>MRGSHHHHHHGSDQVSLGVVGIGKIARDQHLPAIDAEPGFKLTACASRHAEVTGVRNYRDLRALLAAERELDAV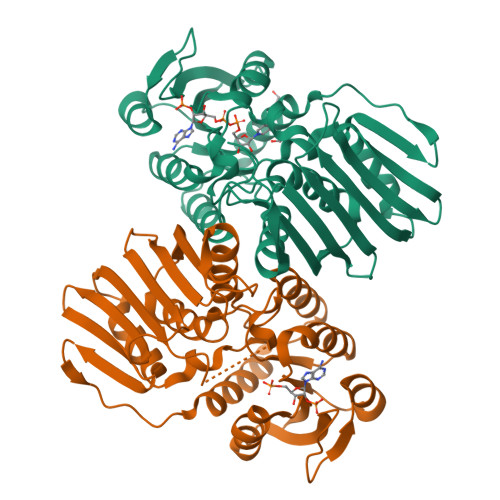SLCAPPQVRYAQARAALEAGKHVMLEKPPGATLGEVAVLEALARERGLTLFATWHSRCASAVEPAREWLATRAIRAVQVRWKADVRRWHPGQQWIWEPGGLGVFDPGINALSIVTRILPRELVLREATLIVPSDVQTPIAAELDCADTDGVPVRAEFDWRHGPVEQWEIAVDTADGVLAISRGGAQLSIAGEPVELGPEREYPALYAHFHALIARGESDVDVRPLRLVADAFLFGRRVQTDAFGR[4x]> SIDSALNWDGEMTVTRFDKMTGAHFVIRLDSTQLGPAAGGTRAAQYSQLADALTDAGKLAGAMTLKMAVSNLPMGGGKSVIALPAPRHSIDPSTWARILRIHAENIDKLSGNYWTGPDVNTNSADMDTLNDTTEFVFGRSLERGGAGSSAFTTAVGVFEAMKATVAHRGLGSLDGLTVLVQGLGAVGGSLASLAAEAGAQLLVADTDTERVAHAVALGHTAVALEDVLSTPCDVFAPCAMGGVITTEVARTLDCSVVAGAANNVIADEAASDILHARGILYAPDFVANAGGAIHLVGREVL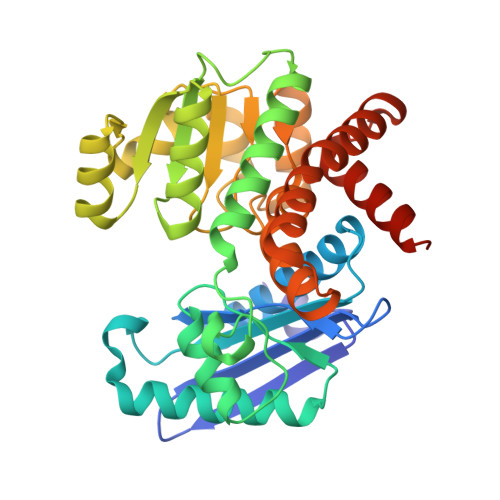GWSESVVHERAVAIGDTLNQVFEISDNDGVTPDEAARTLAGRRAREASTTTATA>[12x]MGSHHHHHHGSLSKFKRNKHQQHLAQLPKISQSVDDVDFFYAPADFRETLLEKIASAKQRI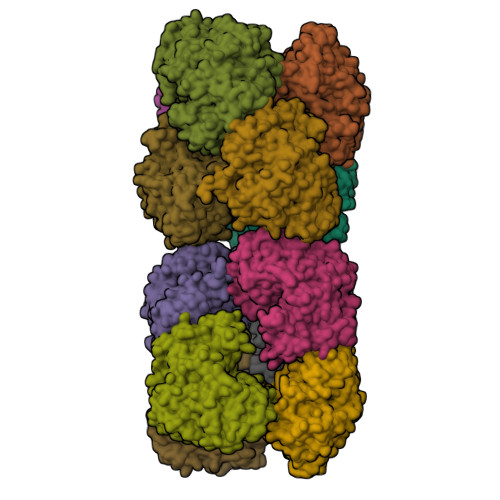CIVALYLEQDDGGKGILNALYEAKRQRPELDVRVLVDWHRAQRGRIGAAASNTNADWYCRMAQENPGVDVPVYGVPINTREALGVLHFKGFIIDDSVLYSGASLNDVYLHQHDKYRYDRYHLIRNRKMSDIMFEWVTQNIMNGRGVNRLDDVNRPKSPEIKNDIRLFRQELRDAAYHFQGDADNDQLSVTPLVGLGKSSLLNKTIFHLMPCAEQKLTICTPYFNLPAILVRNIIQLLREGKKVEIIVGDKTANDFYIPEDEPFKIIGALPYLYEINLRRFLSRLQYYVNTDQLVVRLWKDDDNTYHLKGMWVDDKWMLITGNNLNPRAWRLDLENAILIHDPQLELAPQREKELELIREHTTIVKHYRDLQSIADYPVKVRKLIRRLRRIRIDRLISRIL>VHPITYYPVDTQRLVRSNAERIRHKPYAHYFNPDVAVPEEVFAALKAPLEPEQVLGTSSTELNRLLEPGYLEGETGYCGLPDGAGYTSSLVRFPGATPEMFRWWFWWHSFEPERYSLWHPWCHADIW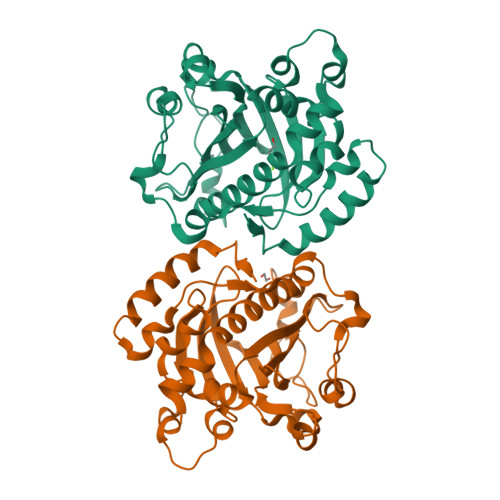RTDPETETAPNLTDEQRYVGSTHHINEYIGQDPLDIEITFIDPARWGFDADGFAAAGIGAHACGSVLMKGSHMRLATMVHLARITDDGFELRSRYWIADRAEPRHDPVAGIAQLTTVPGFSGERQAYEQLVHDQTEFNHLATFLPDIYQEFGP[2x]> SVLLLDVTPLSLGIETMGGVMTTLIAKNTTIPTKHSQVFSMGGAVTIHVLQGERKRAADNKSLGQFNLDGINPAPRGMPQIEVTFDIDADGILHVSAKDKNSGKEQKITIKASSGLNEDEIQKMVRDAEANAEADRKFEELVQT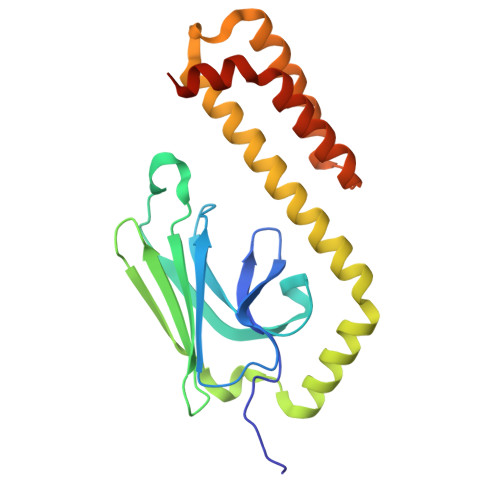RNQGDHLLHSTRKQVEEAGDKLPADDKTAIESALTALETALKGEDKAAIEAKMQELAQVSQKLMEIAQQQHAQQQHA>[2x]AESLPDLKIEKLDEGVYVHTSFEEVNGWGVVPKHGLVVLVNAEAYLIDTPFTAKD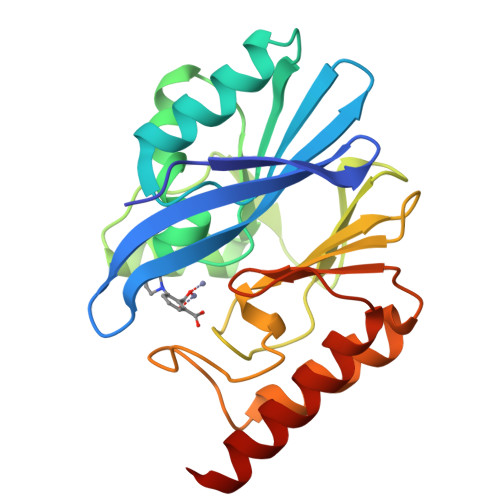TEKLVTWFVERGYKIKGSISSHFHSDSTGGIEWLNSRSIPTYASELTNELLKKDGKVQATNSFSGVNYWLVKNKIEVFYPGPGHTPDNVVVWLPERKILFGGCFIKPYGLGNLGDANIEAWPKSAKLLKSKYGKAKLVVPSHSEVGDASLLKLTLEQAVKGLNESKK> T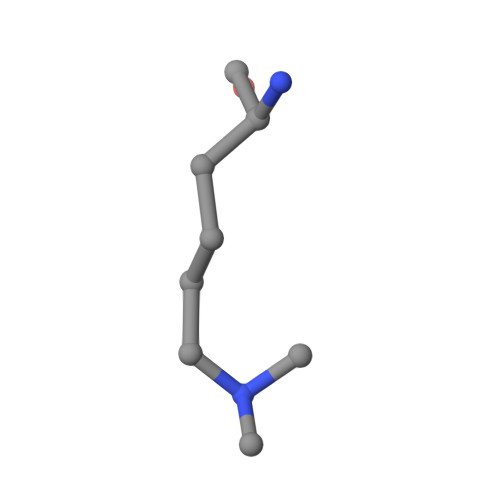SRHKKLMFKT BIS-1,2-{[(Z)-2-CARBOXY-2-METHYL-1,3-DIOXANE]-5-YLOXYCARBAMOYL}-ETHANE | C16 H24 N2 O12 | 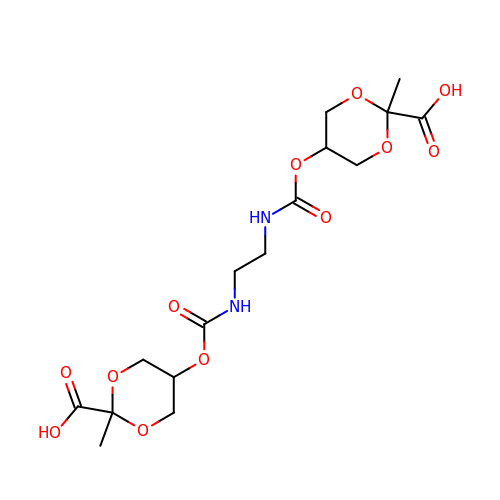HAVIIPIIAVTNFO-GXZHHNFCSA-N> VGVKPVGSDPDFQPELSGAGSRLAVVKFTMRGCGPCLRIAPAFSSMSNKYPQAVFLEVDVHQCQGTAATNNISATPTFQFFRNKVRIDQYQGADA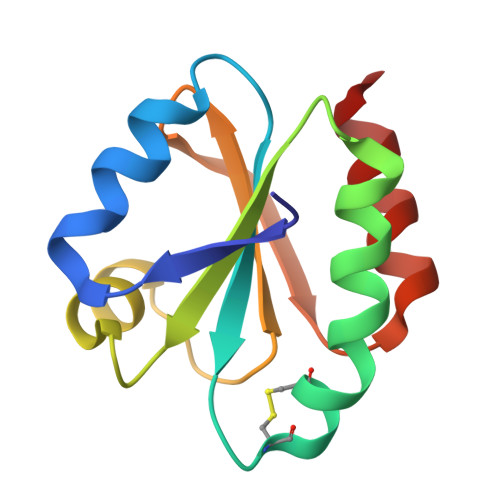VGLEEKIKQHLE>LVPRGSHMKTKMSFGEALEVLKQGMQVYRSGWNGKNMFLFLKSSDALASDFGFGFGEYINEPVFGNIIFIKTADNKIHAWVPSQT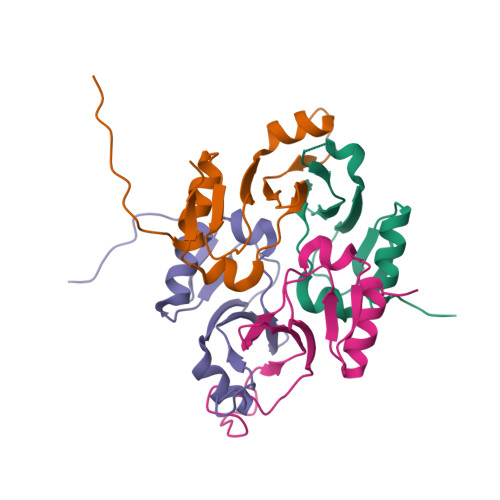DVLAEDWDIVS[6x]>GHMNQIDRLLTIMQRLRDPENGCPWDKEQTFATIAPYTLEETYEVLDAIAREDFDDLRGELGDLLFQVVFYAQMAQEEGRFDFNDICAAISDKLERRHPHVF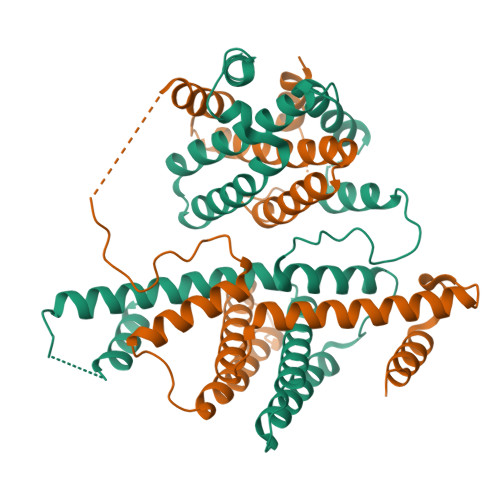ADSSAENSSEVLARWEQIKTEERAQKAQHSALDDIPRSLPALMRAQKIQKRCANVGFDWTTLGPVVDKVYEEIDEVMYEARQAVVDQAKLEEEMGDLLFATVNLARHLGTKAEIALQKANEKFERRFREVERIVAARGLEMTGVDLETMEEVWQQVKRQEIDL[2x]> TVAYIAIGSNLASPLEQVNAALKALGDIPESHILTVSSFYRTPPLGPQDQPDYLNAAVALETSLAPE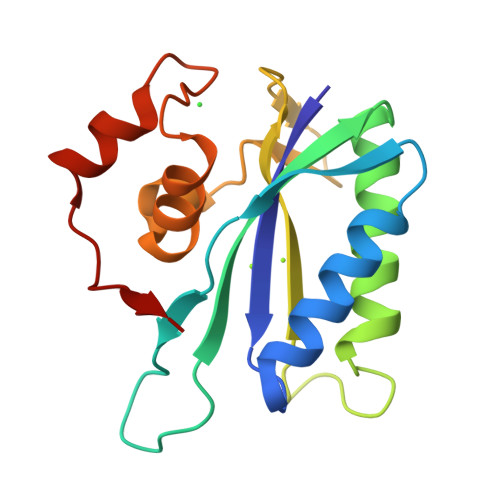ELLNHTQRIELQQGRVRKAERAGPRTLDLDIMLFGNEVINTERLTVPHYDMKNRGFMLWPLFEIAPELVFPDGEMLRQILHTRAFDKLNKW> MISQSRYIRIISGVGAAAPVAGRKLILRVMTT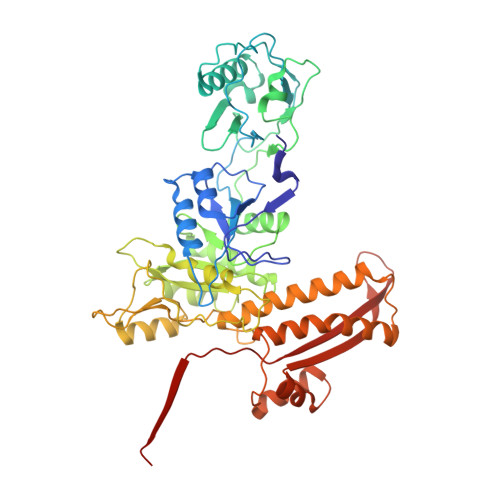NNVIPPGIVIEFDNANAVLSYFGAQSEEYQRAAAYFKFISKSVNSPSSISFARWVNTAIAPMVVGDNLPKTIADFAGFSAGVLTIMVGAAEQNITAIDTSAATSMDNVASIIQTEIRKNADPQLAQATVTWNQNTNQFTLVGATIGTGVLAVAKSADPQDMSTALGWSTSNVVNVAGQSADLPDAAVAKSTNVSNNFGSFLFAGAPLDNDQIKAVSAWNAAQNNQFIYTVATSLANLGTLFTLVNGNAGTALNVLSATAANDFVEQCPSEILAATNYDEPGASQNYMYYQFPGRNITVSDDTVANTVDKSRGNYIGVTQANGQQLAFYQRGILCGGPTDAVDMNVYANEIWLKSAIAQALLDLFLNVNAVPASSTGEAMTLAVLQPVLDKATANGTFTYGKEISAVQQQYITQVTGDRRAWRQVQTLGYWINITFSSYTNSNTGLTEWKANYTLIYSKGDAIRFVEGSDVMI>[2x]GPLGSSNLPVRSFSEVCCAEARAAIIQMENNPDETVCNRIWKIHRDLQSSDLTTTVQVMMVYRFISKRVPEGC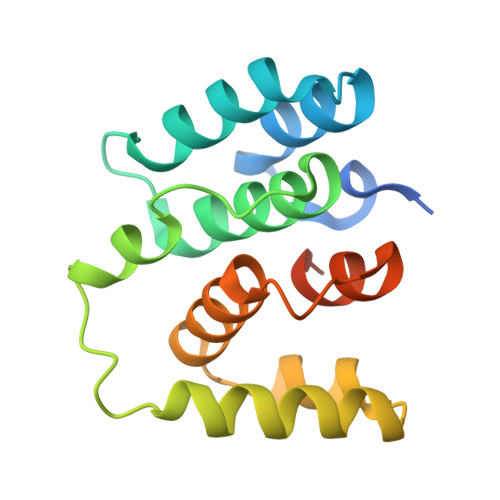FAILSGVNTGMYNPRELKRSYVQSLSSGTSCEFLRSLDKLAKNLLAVHVCSDVKMSLNKRQVIDFISGEEDPTLHTAEHLT>MASDDQWPTFATQGTQFVRDGKPYQVLSGAIHFQRIPRTYWKDRLQKARALGLNTVETYVFWNLVEPQQGQFDFNAN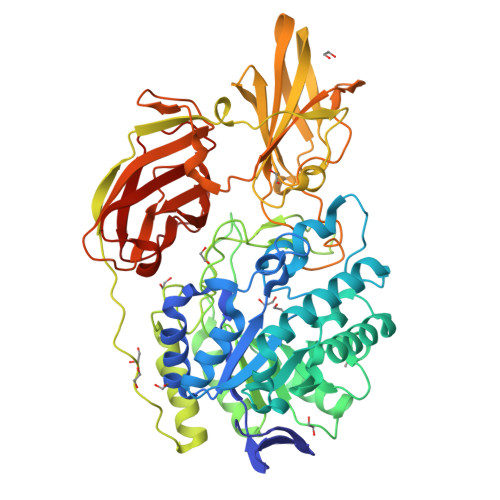NDVAAFVREAAAQGLNVILRPGPYACAEWEAGGYPAWLFGKDNIRIRSRDPRFLAASQSYLDAVAQQVRPLLNHNGGPIIAVQVENEYGSYDDDHAYMADNRAMFVKAGFDKALLFTSDGADMLANGTLPGTLAVVNFAPGEAKSAFDKLIKFQPDQPRMVGEYWAGWFDHWGTPHASTNAKQQTEELEWILRQGHSANLYMFIGGTSFGFMNGANFQGNPSDHYAPQTTSYDYDAILDEAGRPTPKFALMRDVITRVTGVQPPALPAPIAMAALKDAPLRESASLWDNLPAPIAIDTPQPMEHFGQDYGYILYRTTVTGPRKESLYLGEVRDVARVYVDQKPVGSVERRLQQVATEVDIPAGQHTLDVLVENSGRINYGPRMADGRAGLVDPVLLDNQQLTNWQAFPLPMRSPDSIRGWTRNTVEGPAFHRGNLRIGTPADTYLDMRAFGKGIAWANGVNLGRHWNIGPQRALYFPAPFQRKGDNTVVVFDLDSTAKPSVRGLQQQVWITPKE[2x]Here we show that addition of cupric ions to a 6-phosphogluconolactonase 6-PGLac bearing a putative metal binding site leads to the emergence of peroxidase activity (kcat 7.8 × 10–2 s–1, KM 1.1 × 10–5 M). Gratifyingly, this screen revealed one hit: in the presence of CuSO4, 6-phosphogluconolactonase bearing an N131D mutation (Cu·6-PGLac hereafter) catalyzes the oxidation of o-dianisidine (S5 and S6†). Simple metal salt addition thus suffices to endow a protein with novel catalytic activity, very different from the native activity.

Thus, 6-PGLac was co-crystallized with 3 mM CuSO4 followed by soaking with 12 mM CuSO4 (Cu·6-PGLac). The X-ray structure was refined to a resolution of 1.39 Å (Table S4 and Fig. S9†). The third copper (Cu1) is located in the putative metal binding site and displays a T-shaped [2 + 1] coordination geometry. The copper is bound to His67 and His104 (at a distance of 2.00 Å and 1.92 Å, respectively) and displays a weak contact with a water molecule (WATxx 2.80 Å), which is held in place via a hydrogen bond to the carbonyl oxygen of Val101 (O···O 2.81 Å). This structure also contains further unspecifically bound copper ions in the lactonase active site as well as on the surface (Fig. S9C and Table S6†). However, these binding sites are characterized by low occupancy, as reflected by the height of anomalous difference density peaks, and thus presumably have a far lower binding affinity for copper ions. The potentially coordinating oxygen of Asp131 identified by the in silico search and of the Tyr69 are located 6.55 Å and 4.25 Å from Cu1 respectively. Although the STAMPS algorithm suggested a possible facial triad coordination, a T-shaped Cu coordination was observed upon Cu(ii) supplementation.

> ASWSHPQFEKGAMSDTVIERHADTAALVAAAGDRLVDAISSAIGERGQATIVLTGGGTGIGLLKRVRERSGEIDWSKVHIYWGDERFVPQDDDERNDKQAREALLDHIGIPPVNVHAMAASDGEFGDDLEAAAAGYAQLLSADFDSSVPGFDVHLLGMGGEGHVNSLFPDTDAVRETERLVVGVSDSPKPPPRRITLTLPAVQNSREVWLVVSGEAKADAVAAAVGGADPVDIPAAGAVGRERTVWLVDEAAAAKL> GSMGLYFSSLDSSIDILQKRAQELIENINKSRQKDHALMTNFRNSLKTKVSDLTEKLEERIYQIYNDHN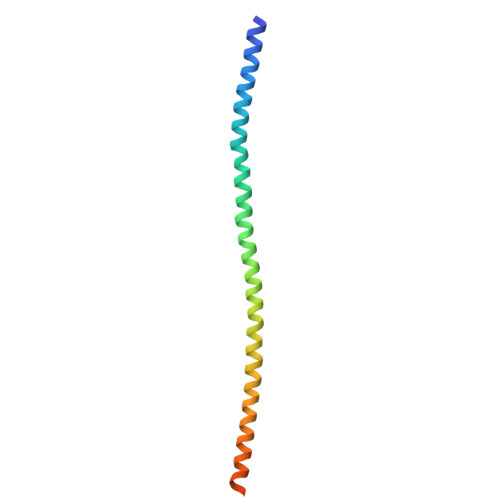KIIQEKLQEFTQKMAKISHLETELKQVCHSVETVYKDLCLQPE> LNDPLDS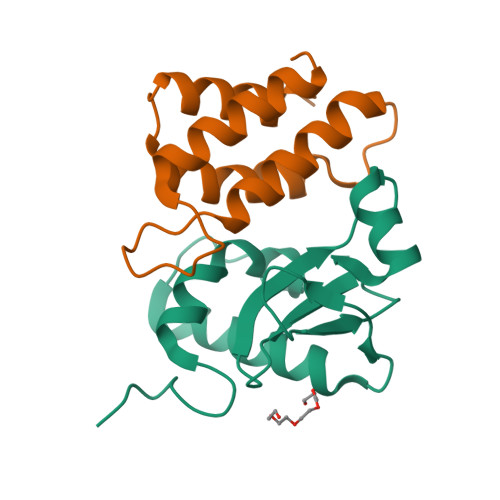GRFSRKQLDKKYKHAGDFGISDTKKNRETLTKFRDAIEEHLSDKDTVEKGTYRREKGSKVYFNPNTMNVVIIKSNGEFLSGWKINPDADNGRIYLETGEL;> MNKMAMIDLAKLFLASKITAIEFSERICVERRRLYGVKDLSPNILNCGEELFMAAERFEPDADRANYEIDDNGLKVEVRSILEKFKL>AHMDQKQFEKIRAVFDRSGVALTLVDMSLPEQPLVLANPPFLRMTGYTEGQILGFNCRFLQRGDENAQARADIRDALKLGRELQVVLRNYRANDEPFDNLLFLHPVGGRPDAPDYFLGSQFELGRSGNSEEAAAAGHAG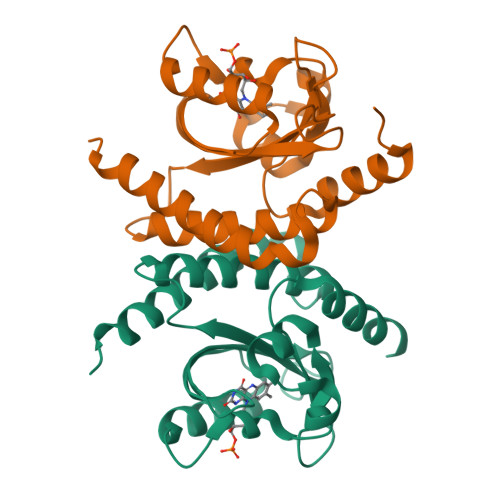ALTGELARIGTVAARLEMDSRRHLAQAAAALVRAWERRG[2x]>MNTPEHMTAVVQRYVAALNAGDLDGIVALFADDATVENPVGSEPRSGTAAIREFYANSLKLPLAVELTQEVRAVANEAAFAFIVSFEYQGRKTVVAPIDHFRFNGAGKV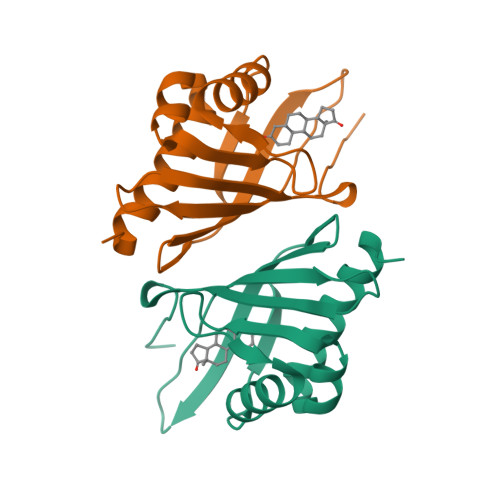VSMRALFGEKNIHAGA[4x]2,3 -ANHYDRO-QUINIC ACID | C7 H10 O5 | 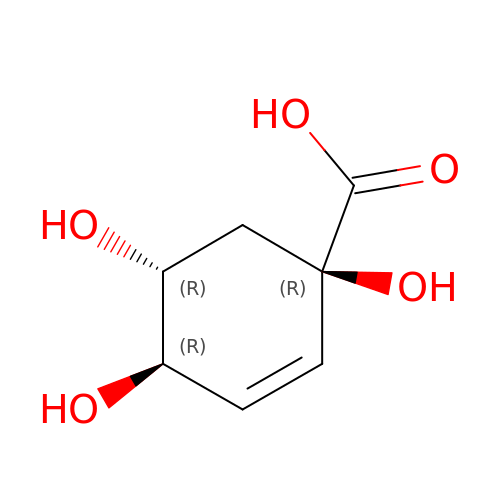VTEDVYGIJPLVFF-XAHCXIQSSA-N> GSHMSTITRPIIELSNTVDKIAEGNLEAEVPHQNRADEIGILAKSIERLRRSLKQLADDRTLLMAGVSHDLRTPLTRIRLATEMMSEQDGYLAESINKDIEECNAIIEQFIDY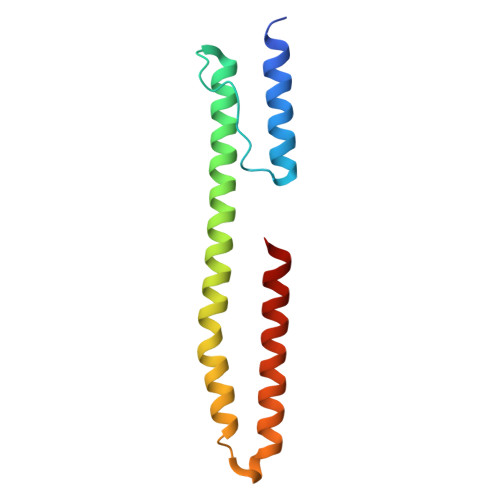LRT2-amino-5-(aminomethyl)-1,7-dihydro-4H-pyrrolo[2,3-d]pyrimidin-4-one 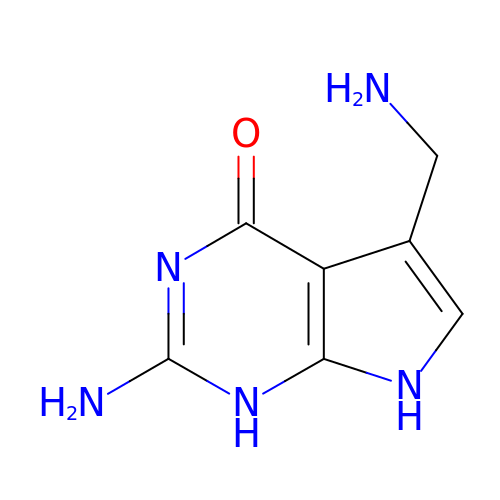| C7 H9 N5 O | MEYMBLGOKYDGLZ-UHFFFAOYSA-N>[4x]MNLKDKILGVAKELFIKNGYNATTTGEIVKLSESSKGNLYYHFKTKENLFLEILNIEESKWQEQWKKEQIKAKTNREKFYLYNELSLTTQYYYP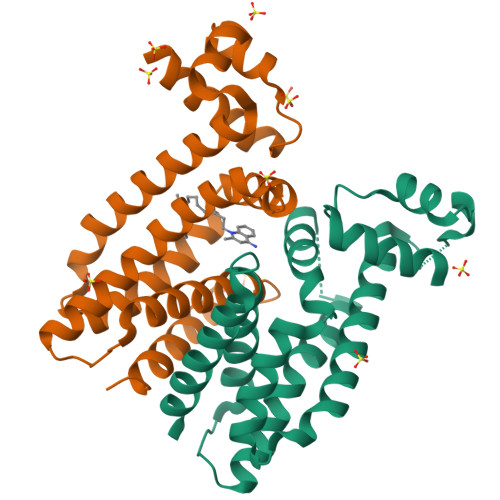LQNAIIEFYTEYYKTNSINEKMNKLENKYIDAYHVIFKEGNLNGEWSINDVNAVSKIAANAVNGIVTFTHEQNINERIKLMNKFSQIFLNGLSKHHHHHH We applied this processing cascade to monoacylglycerol lipase (MAGL), a serine hydrolase that is crucial for the metabolism of neuroprotective endocannabinoid 2-arachidonoylglycerol (2-AG). MAGL represents a target for the development of selective inhibitors aimed at treating central nervous system (CNS) disorders associated with neuroinflammation. For MAGL, an intracellular target, the cellular permeability of inhibitors is a crucial factor for successful drug development.

To confirm and study their binding modes, the co-crystal structures of four inhibitors (17, 23, 27, and 29) with human MAGL were determined. Compared to the human IC50 value of the starting point, hit compound 17 (IC50 = 445 nM), all newly synthesized compounds exhibited enhanced potency. Compared to the binding mode observed for compound 17, the benzoxazole motif on the left side of the molecules is inverted in the new compounds. This flip is likely driven by additional hydrophobic interactions formed by the new substituents in this region of the MAGL binding site. The interactions on the right-hand side of the ligands, including key hydrogen bonds to Met123, Ala51, Arg57, two crystal water molecules, and π-stacking with Tyr194, remain conserved compared to the original hit structure 17. Additionally, an overlay of the three inhibitors (23, 27, and 29) with the hit structure 17 is depicted.

> MGSSHHHHHHSSGENLYFQGMPEESSPRRTPQSIPYQDLPHLVNADGQYLFCRYWAPTGTPKALIFVSHGAGEHSGRYEELARMLMGLDLLVFAHDHVGHGQSEGERMVVSDFHVFVRDVLQHVDSMQKDYPGLPVFLLGHSMGGAIAILTAAERPGHFAGMVLISPLVLANPESATTFKVLAAKVLNSVLPNLSSGPIDSSVLSRNKTEVDIYNSDPLICRAGLKVCFGIQLLNAVSRVERALPKLTVPFLLLQGSADRLCDSKGAYLLMELAKSQDKTLKIYEGAYHVLHKELPEVTNSVFHEINMWVSQRTATAGTASPP> AFYKREMFDPAE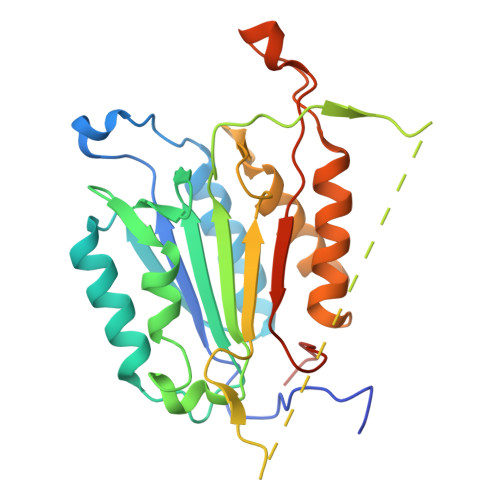KYKMDHRRRGIALIFNHERFFWHLTLPERRGTCADRDNLTRRFSDLGFEVKCFNDLKAEELLLKIHEVSTVSHADADCFVCVFLSHGEGNHIYAYDAKIEIQTLTGLFKGDKCHSLVGKPKIFIIQACRGNQHDVPVIPLDVVDNQTEKLDTNITEVDAASVYTLPAGADFLMCYSVAEGYYSHRETVNGSWYIQDLCEMLGKYGSSLEFTELLTLVNRKVSQRRVDFCKDPSAIGKKQVPCFASMLTKKLHFFPKSNLEHHHHHH>[2x]SFTKFEC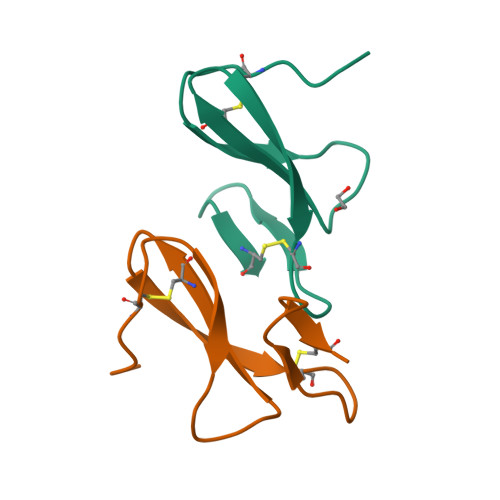PSRFGYFADPKDPHKFYICSNWEAVHKDCPGNTRWNEDEETCT>[3x]MEEVTNVMEYEAIAKKKLPKMVFDYYASGAEDQWTLAENRNAFSRILFRPRILIDVSKIDMSTTVLGFKISMPIMIAPTAMQKMAHPEGEYATARAASAAGTIMTLSSWATSSVEEVASTGPGIRFFQLYVYKDRNVVAQLVRRAERAGFKAIALTVDTPRLGRR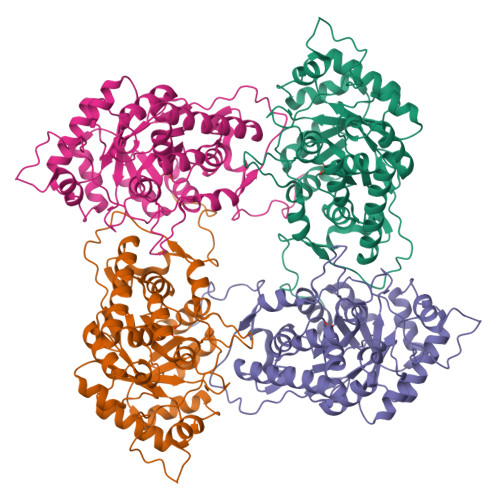EADIKNRFVLPPFLTLKNFEGLDLGKMDQASDSGLASYVAGQIDRTLSWKDVQWLQTITSLPILVKGVLTAEDARLAVQAGAAGIIVSNHGARQLDYVPSTIMALEEVVKAAQGRIPVFLDGGVRRGTDVFKALALGASGIFIGRPVVFSLAAEGEAGIKKVLQMLRDEFELTMALSGCRSLNEITRNHIVTEWDAPRAALPAPRL> GSHMSGIALSRLAQERKAWRKDHPFGFVAVPTKNPDGTMNLMNWECAIPGKKGTPWEGGLFKLRMLFKDDYPSSPPKCKFEPPLFHPNVYPSGTVCLSILEEDKDWRPAITIKQILLGIQELLNEPNIQDPAQAEAYTIYCQNRVEYEKRVRAQAKKFAPS;> STGEPAPVLSSPPPADVSTFLAFPSPEKLLRLGPKSSVLIAQQTDTSDPEKVVSAFLKVSSVFKDEATVRMAVQD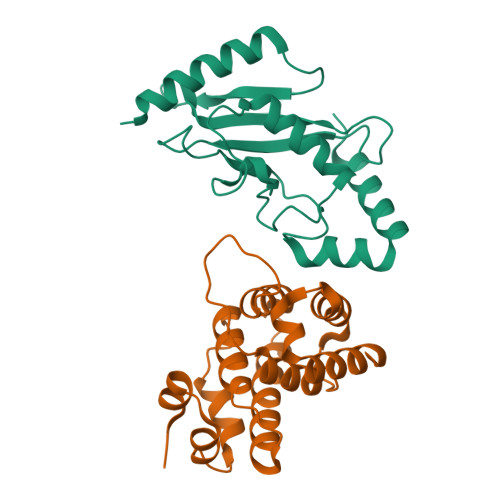AVDALMQKAFNSSSFNSNTFLTRLLVHMGLLKSEDKVKAIANLYGPLMALNHMVQQDYFPKALAPLLLAFVTKPNSALESCSFARHSLLQTLYKV>MMPIKSIVTLDQLEDSEYLFRIVSTVLPHLCLDYKVCDQLKTTFVHPFDILLNNSLGSVTKQDELQAAISKLGINYLIDTTSRELKLFNVT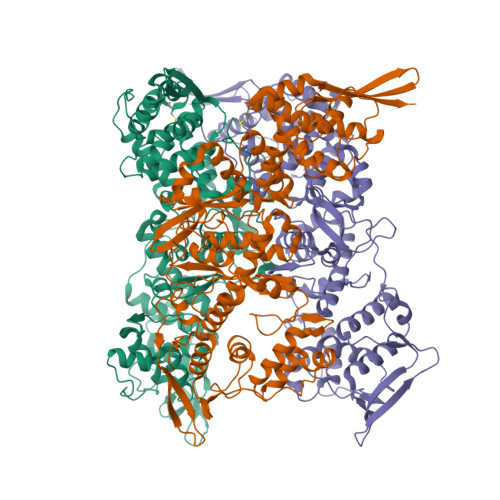LNAGNIDIINTPINISSETNPIINTHSFYDLPPFTQHLLNIRLTDTEYRARFIGGYIKPDGSDSMDVLAEKKYPDLNFDNTYLFNILYKDVINAPIKEFKAKIVNGVLSRQDFDNLIGVRQYITIQDRPRFDDAYNIADAARHYGVNLNTLPLPNVDLTTMPTYKHLIMFEQYFIYTYDRVDIYYNGNKMLFDDEIINFTISMRYQSLIPRLVDFFPDIPVNNNIVLHTRDPQNAAVNVTVALPNVQFVDINRNNKFFINFFNLLAKEQRSTAIKVTKSMFWDGMDYEEYKSKNLQDMMFINSTCYVFGLYNHNNTTYCSILSDIISAEKTPIRVCLLPRVVGGKTVTNLISETLKSISSMTIREFPRKDKSIMHIGLSETGFMRFFQLLRLMADKPHETAIKEVVMAYVGIKLGDKGSPYYIRKESYQDFIYLLFASMGFKVTTRRSIMGSNNISIISIRPRVTKQYIVATLMKTSCSKNEAEKLITSAFDLLNFMVSVSDFRDYQS[3x]> SADERQ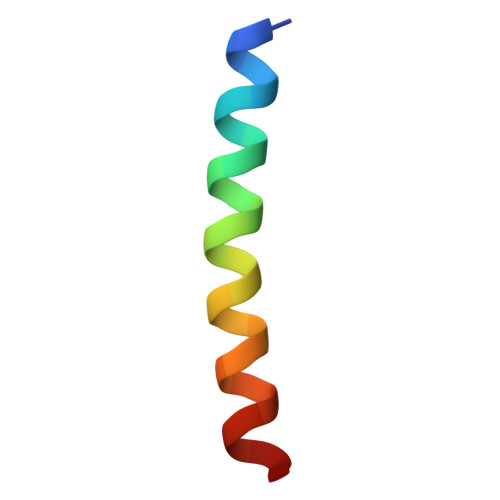RMLVQRKDELLQQARKRFLNK> MAKVVCVLYDDPINGYPTSYARDDLPRIDKYPDGQTLPTPKAIDFTPGALLGSVSGELGLRKYLESQGHELVVTSSKDGPDSELEKHLHDAEVIISQPFWPAYLTAERIAKAPKLKLALTAGIGSDHVDLQAAIDNNITVAEVTYCNSNSVAEHVVMMVLGLVRNYIPSHDWARNGGWNIADCVARSYDVEGMHVGTVAAGRIGLRVLRLLAPFDMHLHYTDRHRLPEAVEKELNLTWHATREDMYGACDVVTLNCPLHPET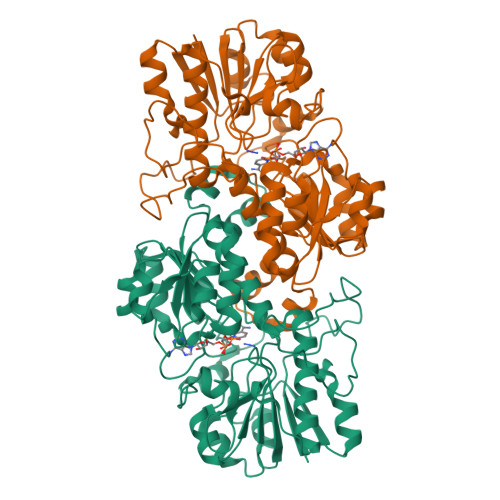EHMINDETLKLFKRGAYLVNTARGKLCDRDAIVRALESGRLAGYAGDVWFPQPAPNDHPWRTMPHNGMTPHISGTSLSAQTRYAAGTREILECYFEGRPIRDEYLIVQGGGLAGVGAHSYSKGNATGGSEEAAKYEKLDA>[4x]GAMDYTLRKIKIAAAHSLSLGLLPTIVKQMPTQFTYAVEAIDVDQAVDMLREGQSDFIFSYHD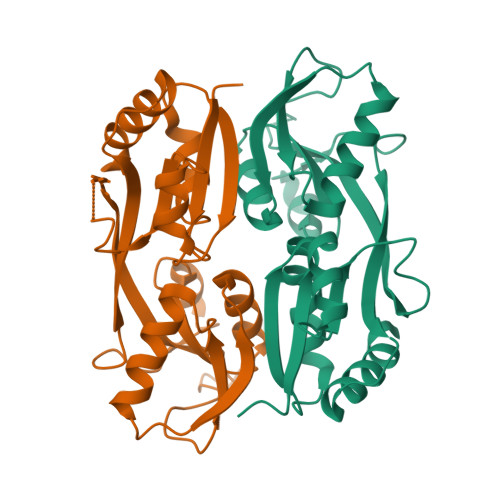ENLQQAPFDNIRLFESRLFPVCANNGRGEPRYTLEQPHFPLLNYSQNSYQGRLINRTLTRHAELSFSTFFVSSMSELLKQVAMDGCGIAWLPEYAIRQEITDGRLIVLDADELVIPIQAYAYRMNTRMSQVAETFWRDLRGLQAAL>[2x]MLDSKLKAPVFTVRTQGREYGEFVLEPLERGFGVTLGNPLRRILLSSIPGTAVTSVYIEDVLHEFSTIPGVKEDVVEIILNLKELVVRFLNPSLQTVTLLLKAEGPKEVKARDFLPVADVEIMNPDLHIATLEEGGRLNMEVRVDRGVGYVPAEKHGIKDRINAIPVDAVFSPVRRVAFQVEDTRLGQRTDLDKLTLRIWTDGSVTPLEALNQAVEILREHLTYFSNPQAAAVAAPEEAKEPEAPPEQEEELDLPLEELGLSTRVLHSLKEEGIESVRALLALNLKDLKNIPGIGERSLEEIKEALEKKGFTLKE;> MEIKRFGRIREVIPLPPLTEIQVESYRRALQADVPPEKRENVGIQAAFRETFPIEEEDKGKGGLVLDFLEYRLGEPPFPQDECREKDLTYQAPLYARLQLIHKDTGLIKEDEVFLGHIPLMTEDGSFIINGADRVIVSQIHRSPGVYFTPDPARPGRYIASIIPLPKRGPWIDLEVEPNGVVSMKVNKRKFPLVLLLRVLGYDQETLARELGAYGELVQGLMDESVFAMRPEEALIRLFTLLRPGDPPKRDKAVAYVYGLIADPRRYDLGEAGRYKAEEKLGIRLSGRTLARFEDGEFKDEVFLPTLRYLFALTAGVPGHEVDDIDHLGNRRIRTVGELMTDQFRVGLARLARGVRERMLMGSEDSLTPAKLVNSRPLEAAIREFFSRSQLSQFKDETNPLSSLRHKRRISALGPGGLTRERAGFDVRDVHRTHYGRICPVETPEGANIGLITSLAAYARVDELGFIRTPYRRVVGGVVTDEVVYMTATEEDRYTIAQANTPLEGNRIAAERVVARRKGEPVIVSPEEVEFMDVSPKQVFSVNTNLIPFLEHDDANRALMGSNMQTQAVPLIRAQAPVVMTGLEERVVRDSLAALYAEEDGEVAKVDGNRIVVRYEDGRLVEYPLRRFYRSNQGTALDQRPRVVVGQRVRKGDLLADGPASENGFLALGQNVLVAIMPFDGYNFEDAIVISEELLKRDFYTSIHIERYEIEARDTKLGPERITRDIPHLSEAALRDLDEEGVVRIGAEVKPGDILVGRTSFKGESEPTPEERLLRSIFGEKARDVKDTSLRVPPGEGGIVVRTVRLRRGDPGVELKPGVREVVRVYVAQKRKLQVGDKLANRHGNKGVVAKILPVEDMPHLPDGTPVDVILNPLGVPSRMNLGQILETHLGLAGYFLGQRYISPIFDGAKEPEIKELLAQAFEVYFGKRKGEGFGVDKREVEVLRRAEKLGLVTPGKTPEEQLKELFLQGKVVLYDGRTGEPIEGPIVVGQMFIMKLYHMVEDKMHARSTGPYSLITQQPLGGKAQFGGQRFGEMEVWALEAYGAAHTLQEMLTLKSDDIEGRNAAYEAIIKGEDVPEPSVPESFRVLVKELQALALDVQTLDEKDNPVDIFEGLASKR;> MKKEVRKVRIALASPEKIRSWSYGEVEKPETINYRTLKPERDGLFDERIFGPIKDYECACGKYKRQRFEGKVCERCGVEVTKSIVRRYRMGHIELATPAAHIWFVKDVPSKIGTLLDLSATELEQVLYFSKYIVLDPKGAILNGVPVEKRQLLTDEEYRELRYGKQETYPLPPGVDALVKDGEEVVKGQELAPGVVSRLDGVALYRFPRRVRVEYVKKERAGLRLPLAAWVEKEAYKPGEILAELPEPYLFRAEEEGVVELKELEEGAFLVLRREDEPVATYFLPVGMTPLVVHGEIVEKGQPLAEAKGLLRMPRQVRAAQVEAEEEGETVYLTLFLEWTEPKDYRVQPHMNVVVPEGARVEAGDKIVAAIDPEEEVIAEAEGVVHLHEPASILVVKARVYPFEDDVEVSTGDRVAPGDVLADGGKVKSDVYGRVEVDLVRNVVRVVESYDIDARMGAEAIQQLLKELDLEALEKELLEEMKHPSRARRAKARKRLEVVRAFLDSGNRPEWMILEAVPVLPPDLRPM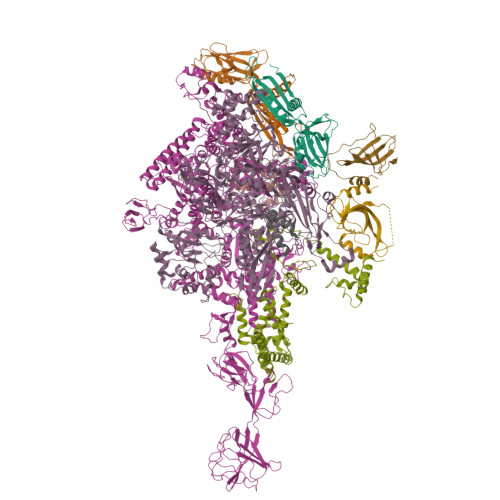VQVDGGRFATSDLNDLYRRLINRNNRLKKLLAQGAPEIIIRNEKRMLQEAVDALLDNGRRGAPVTNPGSDRPLRSLTDILSGKQGRFRQNLLGKRVDYSGRSVIVVGPQLKLHQCGLPKRMALELFKPFLLKKMEEKGIAPNVKAARRMLERQRDIKDEVWDALEEVIHGKVVLLNRAPTLHRLGIQAFQPVLVEGQSIQLHPLVCEAFNADFDGDQMAVHVPLSSFAQAEARIQMLSAHNLLSPASGEPLAKPSRDIILGLYYITQVRKEKKGAGLEFATPEEALAAHERGEVALNAPIKVAGRETSVGRLKYVFANPDEALLAVAHGIVDLQDVVTVRYMGKRLETSPGRILFARIVAEAVEDEKVAWELIQLDVPQEKNSLKDLVYQAFLRLGMEKTARLLDALKYYGFTFSTTSGITIGIDDAVIPEEKKQYLEEADRKLLQIEQAYEMGFLTDRERYDQILQLWTETTEKVTQAVFKNFEENYPFNPLYVMAQSGARGNPQQIRQLCGLRGLMQKPSGETFEVPVRSSFREGLTVLEYFISSHGARKGGADTALRTADSGYLTRKLVDVTHEIVVREADCGTTNYISVPLFQPDEVTRSLRLRKRADIEAGLYGRVLAREVEVLGVRLEEGRYLSMDDVHLLIKAAEAGEIQEVPVRSPLTCQTRYGVCQKCYGYDLSMARPVSIGEAVGIVAAQSIGEPGTQLTMRTFHTGGVAGAADITQGLPRVIELFEARRPKAKAVISEIDGVVRIEETEEKLSVFVESEGFSKEYKLPKEARLLVKDGDYVEAGQPLTRGAIDPHQLLEAKGPEAVERYLVEEIQKVYRAQGVKLHDKHIEIVVRQMMKYVEVTDPGDSRLLEGQVLEKWDVEALNERLIAEGKTPVAWKPLLMGVTKSALSTKSWLSAASFQNTTHVLTEAAIAGKKDELIGLKENVILGRLIPAGTGSDFVRFTQVVDQKTLKAIEEARKEAVEAKERPAARRGVKREQPGKQA;> MAEPGIDKLFGMVDSKYRLTVVVAKRAQQLLRHGFKNTVLEPEERPKMQTLEGLFDDPNAVTWAMKELLTGRLVFGENLVPEDRLQKEMERLYPVEREE;> MKKSKRKNAQAQEAQETEVLVQEEAEELPEFPEGEPDPDLEDPDLTLEDDLLDLPEEGEGLDLEEEEEDLPIPKISTSDPVRQYLHEIGQVPLLTLEEEVELARKVEEGMEAIKKLSEITGLDPDLIREVVRAKILGSARVRHIPGLKETLDPKTVEEIDQKLKSLPKEHKRYLHIAREGEAARQHLIEANLRLVVSIAKKYTGRGLSFLDLIQEGNQGLIRAVEKFEYKRRFKFSTYATWWIRQAINRAIADQARTIRIPVHMVETINKLSRTARQLQQELGREPTYEEIAEAMGPGWDAKRVEETLKIAQEPVSLETPIGDEKDSFYGDFIPDEHLPSPVDAATQSLLSEELEKALSKLSEREAMVLKLRKGLIDGREHTLEEVGAFFGVTRERIRQIENKALRKLKYHESRTRKLRDFLD;>GSHMVEGFVEPYIRLFEAIPDAETELATFYDADLDTLPPRMFLPSGDLYTPPGPVRLEEIKRKRRVRLVKVSIYRFEHVGLGLAARPYAYAYAWQGDNGILHLYHAPVVLEDVPEVLELDEVTYNESYVRLMRAMGHVDAFIDL[2x];> GSHMRTVSVEAIVEALVAEGALRPEEIADFVERITTLDIGTDIFEEQDEGDYWW> MEYRKIQEALEALQKGRL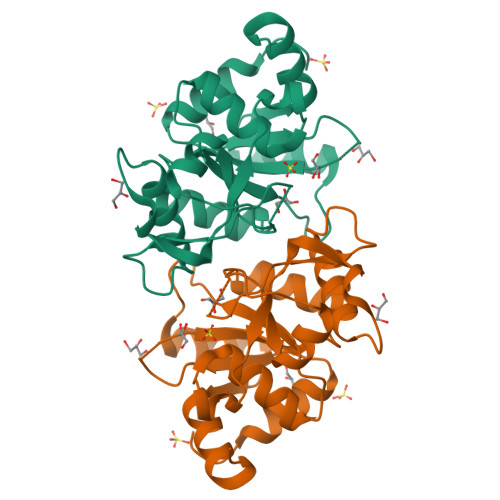VLVIDDKDRENEGDLICSAQAATTENVNFMATYAKGLICMPMSESLANQLMLSPMVENNTDNHKTAFTVSIDYKETTTGISAEERGLTARMCVAEDITPSDFRRPGHMFPLIAKKGGVLERNGHTEATVDLLKLAGLKECGLCCEIMNHDGKMMRTDDLIQFSKKHNIPLITIKELQEYRKVYDQLVERVST> MQNQVDSYRPKLGKKFNEALVFASELHAEQRRKGTEIPYITHLLAVASIIGECGGSEVEVIAGLLHDSVE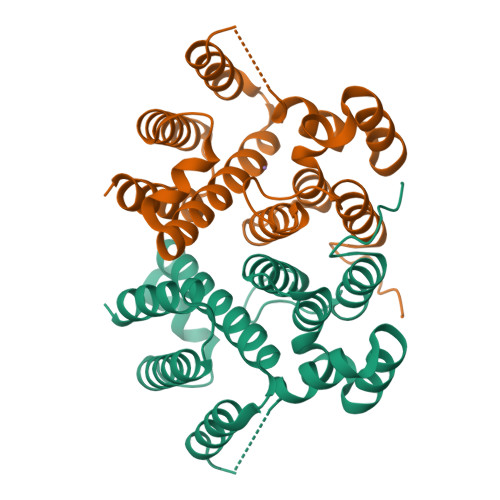DQGGQETLEIIKQKFGNEVAEIVLECSDTDIVPKPPWKERKTAYLNHLKESKNQSVILVSSADKLHNLRSIKSDLSEIGDLVWNRFSASKEETIWYYRELLKIYKVKNAPKRLTIEMEEIIGFIAKLEHHHHHH>[2x]GSSHHHHHHSSGLVPRGSHMLSVGATTTATRLTGWGRTAPS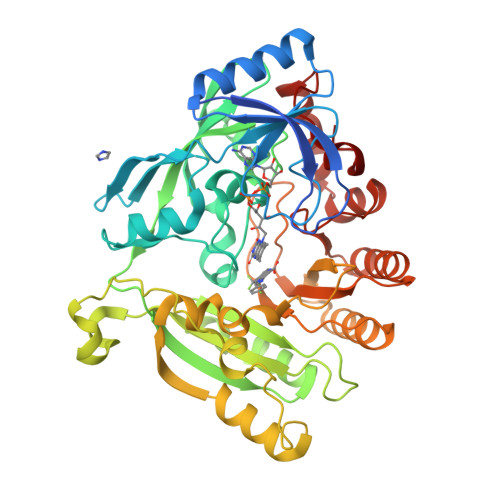VANVLRTPDAEMIVKAVARVAESGGGRGAIARGLGRSYGDNAQNGGGLVIDMTPLNTIHSIDADTKLVDIDAGVNLDQLMKAALPFGLWVPVLPGTRQVTVGGAIACDIHGKNHHSAGSFGNHVRSMDLLTADGEIRHLTPTGEDAELFWATVGGNGLTGIIMRATIEMTPTSTAYFIADGDVTASLDETIALHSDGSEARYTYSSAWFDAISAPPKLGRAAVSRGRLATVEQLPAKLRSEPLKFDAPQLLTLPDVFPNGLANKYTFGPIGELWYRKSGTYRGKVQNLTQFYHPLDMFGEWNRAYGPAGFLQYQFVIPTEAVDEFKKIIGVIQASGHYSFLNVFKLFGPRNQAPLSFPIPGWNICVDFPIKDGLGKFVSELDRRVLEFGGRLYTAKDSRTTAETFHAMYPRVDEWISVRRKVDPLRVFASDMARRLELL> GAKPGKKTRGRVKIKMEFIDNKLRRYTTFSKRKTGIMKKAYELSTLTGT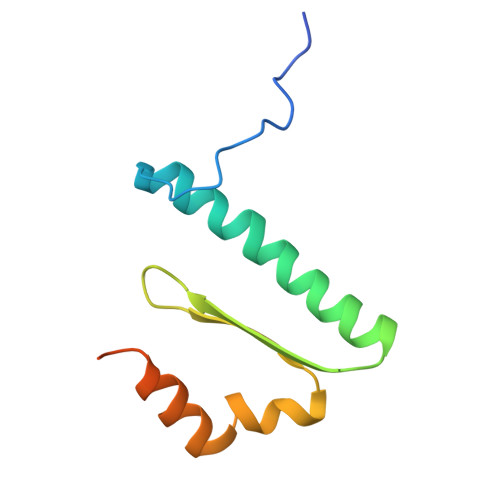QVLLLVASETGHVYTFATRKLQPMITSETGKALIQTCLNSPDSPPRSDPTTDQR methyl [11-oxo-3-(pyridin-4-ylamino)-10,11-dihydro-5H-dibenzo[b,e][1,4]diazepin-8-yl]acetate 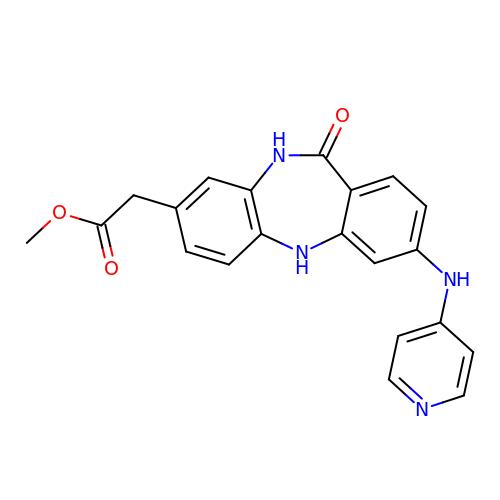| C21 H18 N4 O3 | UHXSMHRHMWNZNO-UHFFFAOYSA-N> QIQKAEQNDVKLAPPTDVRSGYIRLVKNVNYYIDSESIWVDNQEPQIVHFDAVVNLDKGLYVYPEPKRYARSVRQYKILNCANYH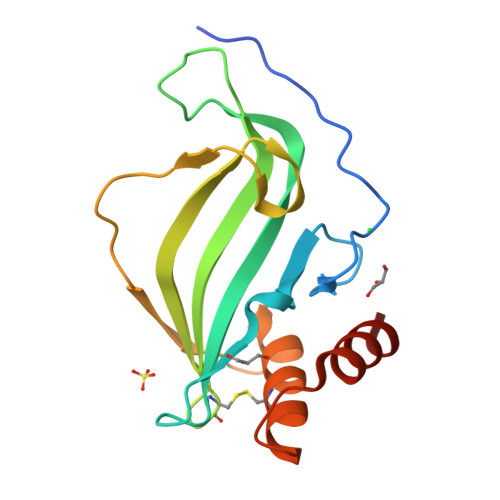LTQVRTDFYDEFWGQGLRAAPKKQKKHTLSLTPDTTLYNAAQIICANYGEAFSVDKKKLAAALEHHHHHH>MRSRILAIVFAARHVAALPLAAEDAAATLSLTSSASSTTVLPSPTQYTLPNNDPNQGARNASIARKRELFLYGPSTLGQTTFYPTGELGNNISARDVLLWRQDAANQTATAYREANETFADITSRGGFKTLDDFALLYNGHWKESVPEGISKGMLSNCTSDLLFSMERLSSNPYVLKRLHPTKDKLPFSVESKVVKKLTATTLEALHKGGRLFLVDHSYQKKYTPQPGRYAAACQGLFYLDARSNQFLPLAIKTNVGVDLTYTPLDDKDDWLLAKIMFNNNDLFYSQMYHVLFHTIPEIVHEAAFRTLSDRHPVMGVLNRLMYQAYAIRPVGGAVLFNPGGFWDQNFGLPASAAIDFPGSVYAQGGGGFQAGYLEKDLRSRGLIGEDSGPRLPHFPFYEDAHRLIGAIRRFMQAFVDSTYGADDGDDGALLRDYELQNWIAEANGPAQVRDFPAAPLRRRAQLVDVLTHVAWITGGAHHVMNQGSPVKFSGVLPLHPAALYAPIPTAKGATGNGTRAGLLAWLPNERQAVEQVSLLARFNRAQVGDRKQTVRDAFAAPDLLAGNGPGYAAANARFVEDTGRISREIAGRGFDGKGLSQGMPFVWTALNPAVNPFFLSV[2x];> AFPISDITVVSERTDASTAYLSDWFVVSFVFSTAGSDETIAGDATIEVSIPNELEFVQYPDSVDPSVSEFFTTAGVQVLSTAFDYDSHVLTFTFSDPGQVITDLEGVVFFTLKLSEQFTESASPGQHTFDFETSDQTYSPSVDLVALDRSQPIKLSNAVTGGVEWFVDIPGAFGDITNIDISTVQTPGTFDCSEVKYAVGSSLNEFGDFTPQDRTTFFSNSSSGEWIPITPASGLPVESFECG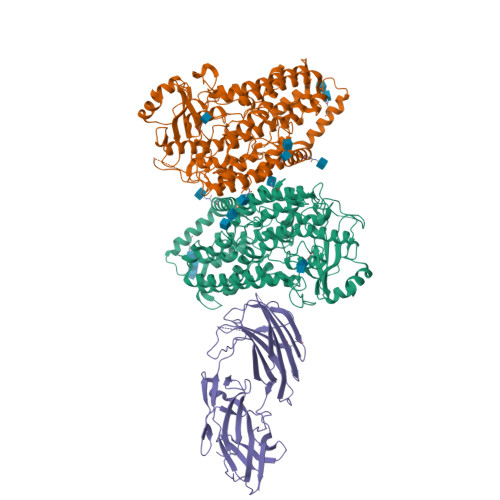DGTISLSFAGELADDEVLRVSFLSNLADDVLEVQNVVNVDLTTADSRKRALTSFVLDEPFYRASRTDTAAFEAFAAV> MSQVTEQSVRFQTALAS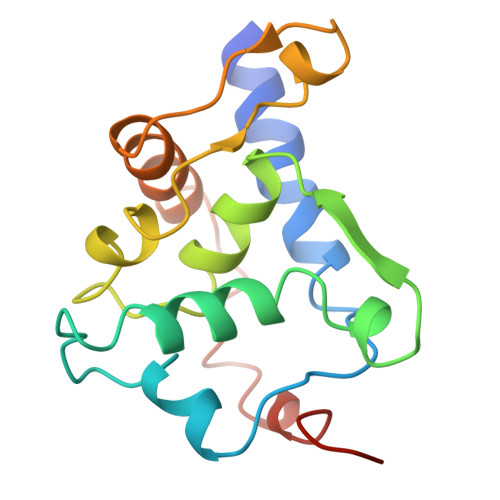IKLIQASAVLDLTEDDFDFLTSNKVWIATDRSRARRCVEACVYGTLDFVGYPRFPAPVEFIAAVIAYYVHPVNIQTACLIMEGAEFTENIINGVERPVKAAELFAFTLRVRAGNTDVLTDAEENVRQKLRAEGVM> GGUGAGG;> CCU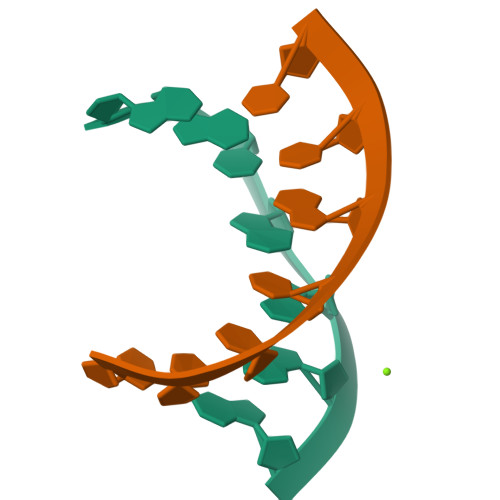CACC>[2x]AG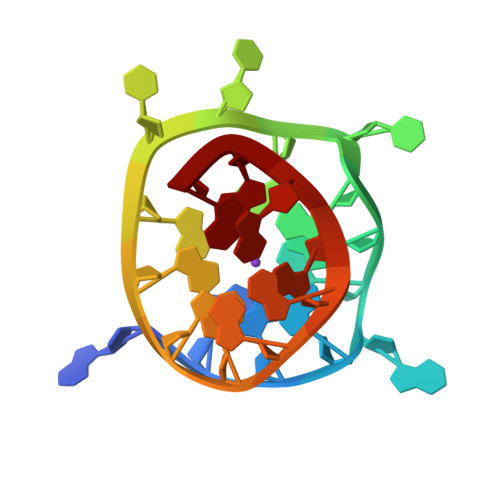GGAGGGCGCTGGGAGGAGGG>HHHHHHMEEEAETEEQQRFSYQQRLKAAVHYTVGCLCEEVALDKEMQFSKQTIAAISELTFRQCENFAKDLEMFARHAKRTTINTEDVKLLARRSNSLLKYITDKSEEIAQIN[4x];>GSHMEGAGAGSGFRKELVSRLLHLHFKDDKTKVSGDALQLMVEL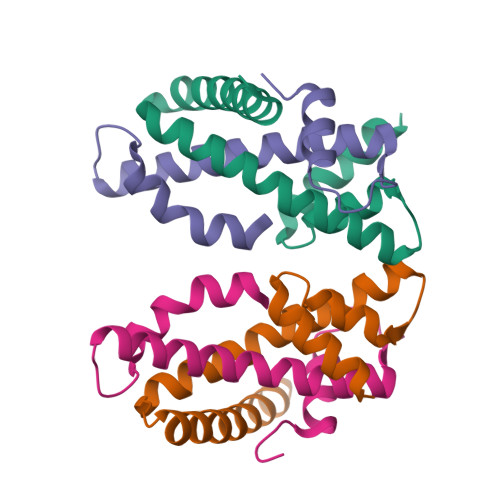LKVFVVEAAVRGVRQAQAEDALRVDVDQLEKVLPQLLLDF[4x]DNA segregation by bacterial ParABS systems is mediated by transient tethering interactions between nucleoid-bound dimers of the ATPase ParA and centromere (parS)-associated complexes of the clamp-forming CTPase ParB. The lifetime of these interactions is limited by the ParB-dependent activation of ParA ATPase activity. We demonstrate that the N-terminal ParA-binding motif of ParB associates with a conserved bipartite binding pocket at the ParA dimer interface, in a manner dependent on ParB clamp closure. Moreover, we show that ParB and non-specific DNA interact cooperatively with ParA and synergistically induce structural changes in its Walker A and Walker B motifs that correlate with the activation of ParA ATPase activity.

However, X-ray analysis revealed that all crystals lacked the peptide and only contained the ParA21-274-D60A•ATP dimer. The structure of the dimeric complex, solved to a resolution of 1.6 Å, was highly similar to that of the H. pylori ParA·ATP dimer35 (RMSD of 0.767 Å for 225 paired Cα atoms), in line with the high functional conservation of the ParABS system among bacteria. The structure of the ParA21-274 dimer in these high-confidence models is similar to the crystal structure of the ParA21-274-D60A•ATP dimer complex (RMSD of 0.527 Å for 242 paired Cα atoms), supporting the general validity of the modeling approach. When associated with ATP, two monomers interact face-to-face, with the nucleotides sandwiched in between the two subunits. In the case of ParA, ATP-bound homodimers have non-specific DNA-binding activity, mediated by clusters of positively charged residues that line the edge of the subunit interface. A combination of computational modeling, nuclear magnetic resonance (NMR) spectroscopy and mutational studies reveals that ParB interacts with a conserved hydrophobic pocket at the edge of the ParA dimer interface that is formed by residues from both subunits and includes a loop immediately adjacent to the deviant Walker A motif of ParA. The fact that the ParB-binding pocket is constituted by amino acids from both ParA subunits explains why the association of ParB can only occur upon ParA dimerization. The ParA dimer contains two ParB-binding sites located face-to-face on opposite sides of the dimer interface. However, there was a noticeable increase in HDX in a region at the catalytic site of ParA comprising the Walker B motif and an adjacent loop that reaches up to the ParB-binding site and contains the essential ParB-interacting residues L150 and L152.

>[2x]GVGRIICISNQKGGVGKTTTAINLAASLASAERRTLLVDMAPQGNAGSGLGIKQDNITGTIYEALLNDRPIQELLHPTELRYLQVVPATPDLTGAEVELVNQDNREFRLRDALRPLAAEYDYIIIDCPPSLGLLTLNALAAADSVLIPLQCEYYALEGLSQLTHTIDLVKQGLNPDLKMEGILLTMFDSRANIAHQVVEEVRGYFKKQVFEVIVPRNVRLSECPSFGKPIILYDIKSKGCESYLALGRELMKRDT> RQLVFLEWHEAPTIAVALLAALGFLSTLAILVIFWRHFQTPIVRSAGGPMCFLMLTLLLVAYMVVPVYVGPPKVSTCLCRQALFPLCFTICISCIAVRSFQIVCAFKMASRFPRAYSYWVRYQGPYVSMAFITVLKMVIVVIGMLATGLSPTTRTDPDDPKITIVSCNPNYRNSLLFNTSLDLLLSVVGFSFAYMGKELPTNYNEAKFITLSMTFYFTSSVSLCTFMSAYSGVLVTIVDLLVTVLNLLAISLG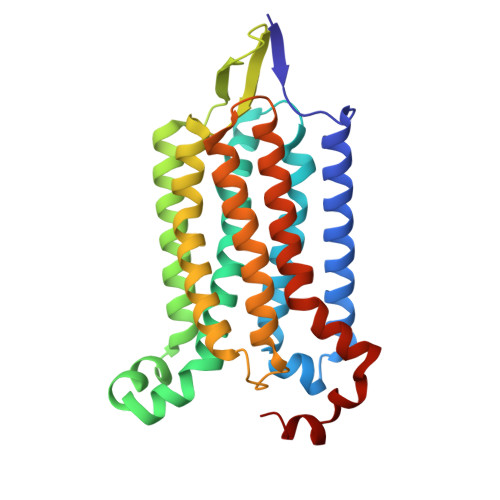YFGPKCYMILFYPERNTPAYFNSMI>MSMILKEIRMNNFKSHVNSRIKFEKGIVAIIGENGSGKSSIFEAVFFALFGAGSNFNYDTIITKGKKSVYVELDFEVNGNNYKIIREYDSGRGGAKLYKNGKPYATTISAVNKAVNEILGVDRNMFLNSIYIKQGEIAKFLSLKPSEKL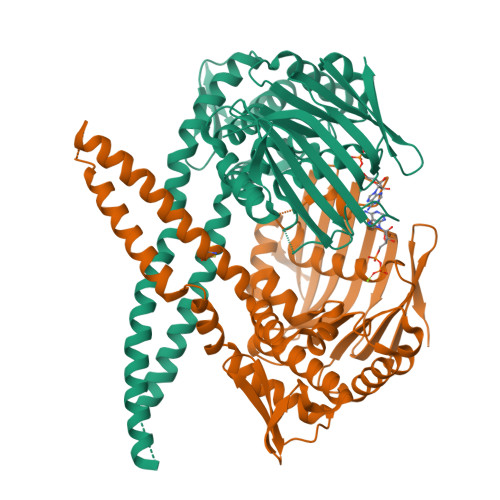ETVAKLLGIDEFEKCYQKMGEIVKEYEKRLERIEGELNYKEESLKARLKEMSNLEKEKEKLTKFVEYLDKVRRIFGRNGFQAYLREKYVPLIQKYLNEAFSEFDLPYSFVELTKDFEVRVHAPNGVLTIDNLSGGEQIAVALSLRLAIANALIGNRVECIILDEPTVYLDENRRAKLAEIFRKVKSIPQMIIITHHRELEDVADVIINVKKDGNVSKVKING[2x]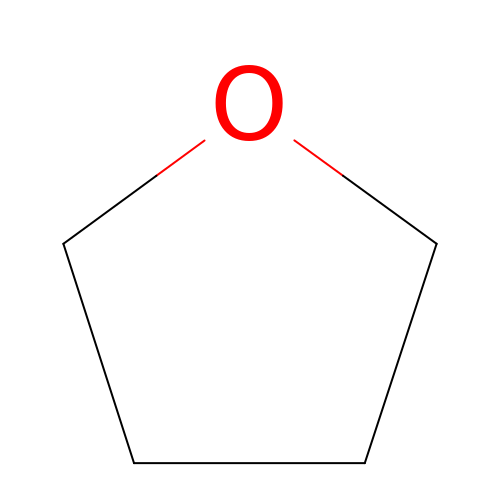tetrahydrofuran | C4 H8 O | WYURNTSHIVDZCO-UHFFFAOYSA-N> QSMTESTVDRINGITPSALDLIGNTPLIALDRLWPGPGRLLAKCEFLNPTASLKDRSSYYMIAKAKESGQLKDGESVIEVTS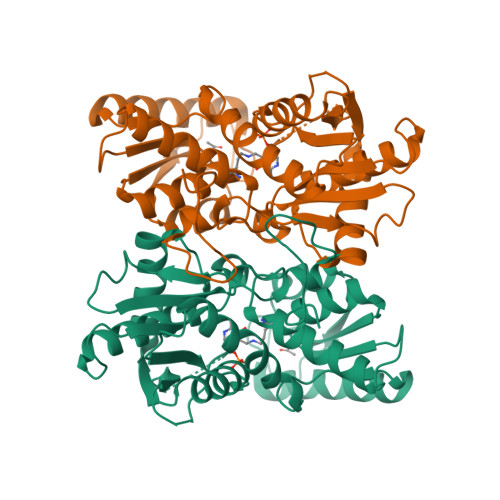GNQGGGIACVTAVMGHPFTVTMSKGNSPQRAIMMNALGANVILVDQVTGKPGNVTADDVAAAEETAMKIREETNAYYVDQFNNPTNCLAHYETTGPEIWRQTNGRIDAFLVGCGTGGCFVGTSKFLKEKNPNVRCFVVEPEGCQPIAGCTITKPLHLLQGSGYGCVPTLFDKKVYNDSISVSDEEAIEYRKLLGQKEGLFCGFTTGGNIAAAIKLLKSGQLPKDAWVVTILCDSGLKYPE>GGGGSMSTAEPAPDPTNPSTSGLAPTTNGIGSPPPTASAATKFSILTKFLRRKNQVHTTTAQQNEFMQKYMPNGNSNAVQPAATGGQPASSDGGSAIEVPPPKESYAVRIRKYLANYTQDPSTDNFYYWTCVVTVAYIYNLLFVIARQVFNDLIGPSSQSLCRFYNGTLNSTTQVECTYNMLTNMKEMPTYSQYPDLGWSKYWHFRMLWVFFDLLMDCVYLIDTFLNYRMGYMDQGLVVREAEKVTKAYWQSKQYRIDGISLIPLDYILGWPIPYINWRGLPILRLNRLIRYKRVRNCLERTETRSSMPNAFRVVVVVWYIVIIIHWNACLYFWISEWIGLGTDAWVYGHLNKQSLPDDITDTLLRRYVYSFYWSTLILTTIGEVPSPVRNIEYAFVTLDLMCGVLIFATIVGNVGSMISNMSAAWTEFQNKMDGIKQYMELRKVSKQLEIRVIKWFDYLWTNKQSLSDQQVLKVLPDKLQAEIAMQVHFETLRKVRIFQDCEAGLLAELVLKLQLQVFSPGDFICKKGDIGREMYIVKRGRLQVVDDDGKKVFVTLQEGSVFGELSILNIAGSKNGNRRTANVRSVGYTDLFVLSKTDLWNALREYPDARKLLLAKGREILKKDNLLDENAPEEQKTVEEIAEHLNNAVKVLQTRMARLIVEHSSTEGKLMKRIE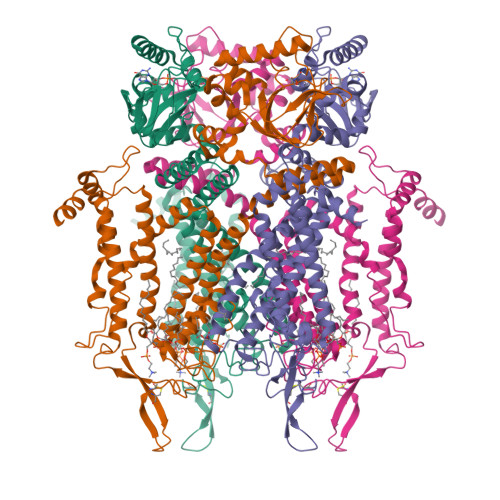MLEKHLSRYKALARRQKTMHGVSIDGGDISTDGVDERVRPPRLRQTKTIDLPTGTESESLLK[4x]>[5x]SYDTVMDKY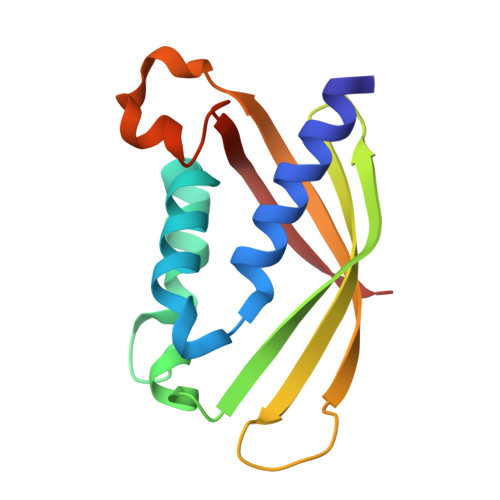WLSQYVIARETYDWYTLQKDYETVGMLSSPSEGQSYASQFQGDKALDKQYGSNVRTSVTIVSIVPNGKGIGTVRFAKTTKRTNETGDGETTHWIATIGYQYVNPSLMSESARLTNPLGFNVTSYRVDPE>[2x]MWLLALCLVGLAGAQRGGGGPGGGAPGGPGLGLGSLGEERFPVVNTAYGRVRGVRRELNNEILGPVVQFLGVPYATPPLGARRFQPPEAPASWPGVRNATTLPPACPQNLHGALPAIMLPVWFTDNLEAAATYVQNQSEDCLYLNLYVPTEDGPLTKKRDEATLNPPDTDIRDPGKKPVMLFLHGGSYMEGTGNMFDGSVLAAYGNVIVATLNYRLGVLGFLSTGDQAAKGNYGLLDQIQALRWLSENIAHFGGDPERITIFGSGAGASCVNLLILSHHSEGLFQKAIAQSGTAISSWSVNYQPLKYTRLLAAKVGCDREDSAEAVECLRRKPSRELVDQDVQPARYHIAFGPVVDGDVVPDDPEILMQQGEFLNYDMLIGVNQGEGLKFVEDSAESEDGVSASAFDFTVSNFVDNLYGYPEGKDVLRETIKFMYTDWADRDNGEMRRKTLLALFTDHQWVAPAVATAKLHADYQSPVYFYTFYHHCQAEGRPEWADAAHGDELPYVFGVPMVGATDLFPCNFSKNDVMLSAVVMTYWTNFAKTGDPNQPVPQDTKFIHTKPNRFEEVVWSKFNSKEKQYLHIGLKPRVRDNYRANKVAFWLELVPHLHNLHTELFTTTTRLPPYATRWPPRPPAGAPGTRRPPPPATLPPEPEPEPGPRAYDRFPGDSRDYSTELSVTVAVGASLLFLNILAFAALYYKRDRRQELRCRRLSPPGGSGSGVPGGGPLLPAAGRELPPEEELVSLQLKRGGGVGADPAEALRPACPPDYTLALRRAPDDVPLLAPGALTLLPSGLGPPPPPPPPSLHPFGPFPPPPPTATSHNNTLPHPHSTTRV

Neuroligins are postsynaptic membrane cell adhesion molecules that connect presynaptic and postsynaptic neurons, mediate the transmission of signals between synapses, and shape the characteristics of neural networks through specific synaptic functions. NLGNs belong to single transmembrane proteins, and they all consist of a large extracellular, acetylcholinesterase-like domain (CLD) and a carbohydrate-binding region, following the transmembrane region of O-glycosylation helix and the C-terminal intracellular region as postsynaptic density zone (PDZ) recognition component, which mainly binds to postsynaptic target proteins such as Gephyrin and postsynaptic density protein, thus promoting synaptic differentiation and strengthening the stability of synaptic space and the function of transmitting intersynaptic signals. The ectodomains of NLGNs can form specific cross-synaptic connections with neurexins (NRXNs) of the presynaptic membrane, and these connections can be regulated by the membrane-associated mucin (MAM) domain-containing glycosylphosphatidylinositol anchor (MDGAs). The NLGN structures were highly conserved in both human NLGN2 and human NLGN3 dimer forms as two symmetrical elliptical spheres, and the interface comprises a four-helix bundle including two helices from each protomer.

NLGN1 is mainly expressed at excitatory synapses, NLGN2 is mainly expressed at inhibitory synapses, NLGN3 is expressed at both excitatory and inhibitory synapses, and NL4 expression seems to be limited to the glycinergic synapses of retinal glial cells and several other regions of the central nervous system. For NLGN2 protomer, it contains an α/β hydrolase fold, a 13-stranded central curved β-sheet surrounded by 22 α-helices. The interface area between NLGN2 dimer is about 744 Å2, which consisted of interacting residues (E429, H607, M434, F433, A599, Q592, L604, A439, W438, and Q596), among which E429 and H607 form salt bridges, and other residues mainly contribute hydrophobic interactions. The extracellular domain of NLGN2 is a cholinesterase-like domain, which might be required for synapse-specific functions. The overall structure of NLGN2 and NLGN3 protomers is very similar, with root-mean-square deviation (RMSD) of 1.518 Å over 522 Cα atoms. However, when chain A from NLGN2 and NLGN3 was superimposed, the orientation of chain B from NLGN3 has a rotation relative to that from NLGN2, indicating the distinct arrangement adopted by different NLGNs. The structural alignment shows that the relative rotation of chain B may affect the interaction between NLGN2 and MDGA1. The interacting residues were mapped to the previously identified patches A–C. The results intuitively showed a slight difference in patch B, where F408 of NLGN2 was substituted by Y431 in NLGN3. Sequence alignment shows that NLGN2 also has the corresponding arginine residue at position 428 in a conserved region.>KETTSFVFTRFSPDPQNLLLQGDTVVTSSGHLQLTQVKDGEPVYSSLGRALYYAPIHIWDSNTDTVANFVTSFSFVIDAPNKAKAADGLAFFLAPVDTEPQKPGGLLGLFHDDRHNKSNHIVAVEFDTFKNSWDPE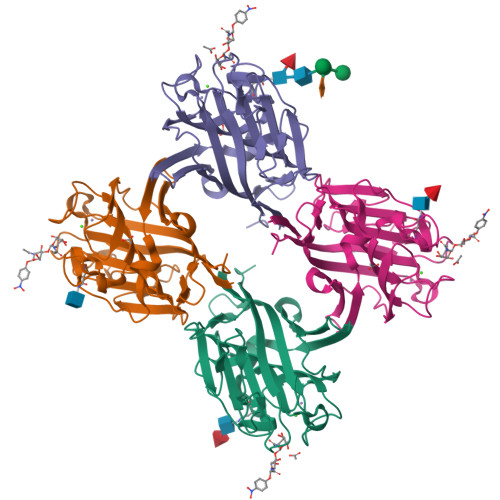GTHIGINVNSIVSRKTISWDLENNEVANVVISYQASTKTLTASLVYPSSSTSYILNDVVDLKQILPEYVRVGFTAASGLSKDHVETHDVLAWTFDSDLPDPSSDDCN[4x]>[4x]MAHHHHHHMTTYTLVLLRHGESTWNKENKFTGWTDVPLSEKGEEEAIAAGKYLKEKNFKFDVVYTSVLKRAICTAWNVLKTADLLHVPVVKTWRLNERHCGSLQGLNKSETAKKYGEEQVKIWRRSYDIPPPKLDKEDNRWPGHNVVYKNVPKDALPFTECLKDTVERVLPFWFDHIAPDILANKKVMVAAHGNSLRGLVKHL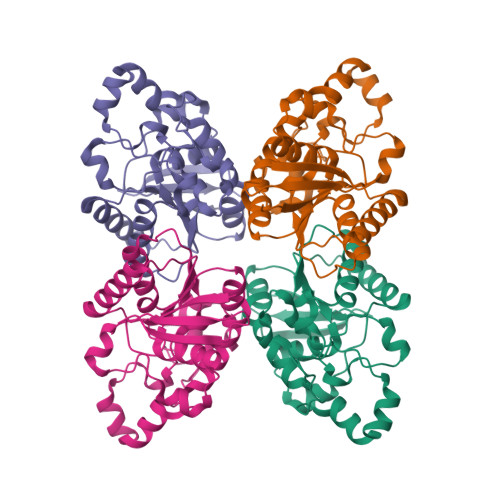DNLSEADVLELNIPTGVPLVYELDENLKPIKHYYLLDSEELKKKMDEVANQGKAK>[2x]TSNVITQDLPIPVASRGFADIVGFGLDGVVIGRNAVNLQPFLAVKNFAQNAGGWLTTKHVRLIADTTGTGKGDIVGFGNAGVYVSVNNGKNTFADPPKMVIANFGYDAGGW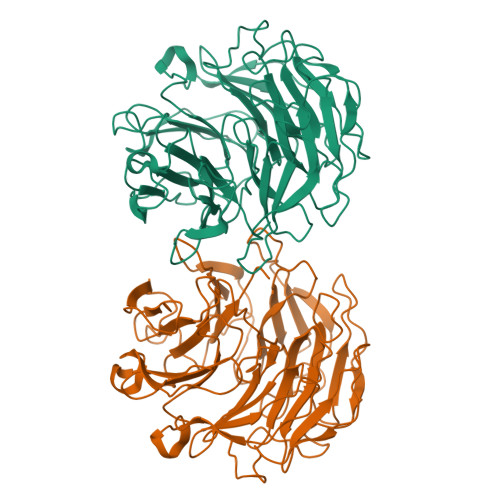RVEKHLRYLADIRKTGRADIIGFGEKGVLVSRNNGGLNFGPATLVLKDFGYDAGGWRLDRHLRFLADVTGNGHLDIVGFGDKHVFISRNNGDGTFAPAKSVIDNFCIDAGGWKIGDHPRFVADLTGDGTADIIGCGKAGCWVALNNGGGVFGQVKLVINDFGTDKGWQAAKHPRFIADLTGNGRGDVVGFGNAGVYVALNNGDGTFQSAKLVLKDFGVQQGWTVSKHRRFVVDLTGDGCADIIGFGEKETLVSYNDGKGNFGPVKALTNDFSFSGGKWAPETTVCWMANLDSSRH>[4x]SYSTLANFPVQARNDNISPWTITGFADAESSFMLTVSKDSKRNTGWSVRPRFRIGLHNKDVTILKSIREYLGAGIITSDIDARIRFESLKELEVVINHFDKYPLITQKRADYLLFKKAFYLIKNKEHLTEEGLNQILTLKASLNLGLSEELKEAFPNTIPAERLLVTGQEIPDSNWVAGFTAAEGSFYIRIAKNSTLKTGYQVQSVFQITQDTRDIELMKNLISYLNCGNIRIRKYKGSEG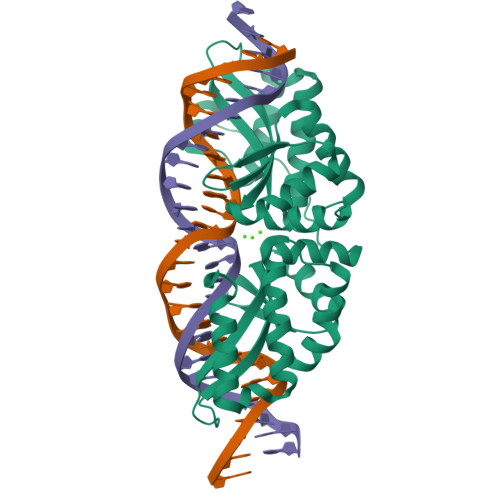IHDTCVDLVVTNLNDIKEKIIPFFNKNHIIGVKLQDYRDWCKVVTLIDNKEHLTSEGLEKIQKIKEGMNRGRSL The replicase (Rep) from these viruses is responsible for initiating rolling circle replication (RCR) of their genomes. Rep is a multifunctional enzyme responsible for nicking and ligating ssDNA and unwinding double-stranded DNA (dsDNA). At the Rep N terminus is an endonuclease domain (ED) that is responsible for ssDNA nicking and ligation, in the center of Rep is an oligomerization domain (OD) responsible for hexamerization, and at the C terminus is an ATPase domain (AD) responsible for ssDNA/dsDNA interaction and translocation. The structures demonstrate Rep to be a member of the superfamily 3 (SF3) of ATPases Associated with diverse cellular Activities (AAA+) superfamily clade 4.

To understand the architecture of Reps from CRESS-DNA viruses and how they interact with dsDNA and ssDNA to unwind dsDNA, we determined the structure of PCV2b Rep bound to ssDNA and dsDNA using cryo-electron microscopy (cryo-EM) to 3.8-Å and 4.4-Å resolution, respectively. The docking reveled that the density could accommodate only ssDNA. The 3′-to-5′ orientation refined to a cross correlation (CC) of 0.64 with a Clashscore of 0.0, and the 5′-to-3′ orientation refined to a CC of 0.5 with a Clashscore of 4.4. The better quality of fit for the 3′-to-5′ orientation independently agrees with the biochemical data demonstrating Rep to exhibit 3′-to-5′ helicase activity. While the density describing the sugar-phosphate backbone of the ssDNA is strong and convincing, the density describing the bases of the nucleic acid is smeared, likely due to conformational and sequence heterogeneity within the data set, and therefore, the modeled poly(dT) is a generalized interpretation of the multiple ssDNA sequences bound to Rep. The backbone phosphates from four consecutive nucleotides interact with the six subunits of Rep (1 nt subunit−1). The phosphates from ssDNA interact with amino acids located in two loops: pore loop 1 located between β2 and α2 (Trp202) and pore loop 2 (also known as the “presensor 1 β-hairpin”) located between α3 and β4 (Lys240 and Gly241). Density for the ssDNA extends toward the center of the OD ring and terminates near the guanidium group of Arg148, suggesting that ssDNA is translocated through the pore. Subunits A (top of staircase) and F (bottom of staircase) make limited interactions with ssDNA, whereas subunits B through E more intimately engage ssDNA. In total, there are seven direct interactions between Rep and ADP in the AB interface, three in the BC interface, two in the CD and DE interface, and no nucleotide present in the EF or FA interfaces.

>MPSKKNGRSGPQPHKRWVFTLNNPSEDERKKIRELPISLFDYFIVGEEGNEEGRTPHLQGFANFVKKQTFNKVKWYFGARCHIEKAKGTDQQNKEYCSKEGNLLMECGAPRSQGQRSDLSTAVSTLLESGSLVTVAEQHPVTFVRNFRGLAELLKVSGKMQKRDWKTNVHVIVGPPGCGKSKWAANFADPETTYWKPPRNKWWDGYHGEEVVVIDDFYGWLPWDDLLRLCDRYPLTVETKGGTVPFLARSILITSNQTPLEWYSSTAVPAVEALYRRITSLVFWKNATEQSTEEGGQFVTLSPPCPEFPYEINY[6x]> SGPRPRLWEGQDVLARWTDGLLYLGTIKKVDSAREVCLVQFEDDSQFLVLWKDISPAALPGEEL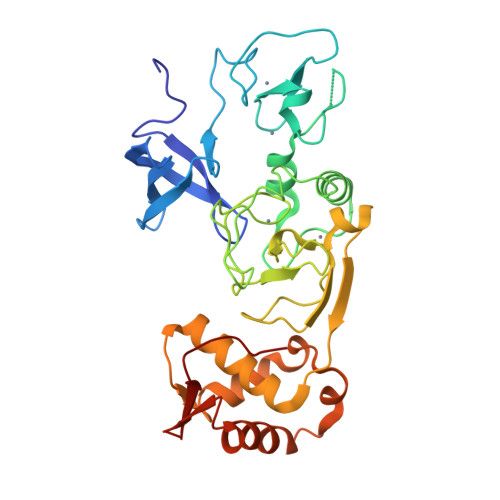LCCVCRSETVVPGNRLVSCEKCRHAYHQDCHVPRAPAPGEGEGTSWVCRQCVFAIATKRGGALKKGPYARAMLGMKLSLPYGLKGLDWDAGHLSNRQQSYCYCGGPGEWNLKMLQCRSCLQWFHEACTQCLSKPLLYGDRFYEFECCVCRGGPEKVRRLQLRWVDVAHLVLYHLSVCCKKKYFDFDREILPFTSENWDSLLLGELSDTPKGERSSRLLSALNSHKDRFISGREIKKRKCLFGLHARMPPPVE> SRMQEKHMRIRVKLLDSTVELFDIEPKCDGQVLLTQVWKHLNLIECDYFGLEFKNVQSYWIWLEPMKPIIRQVRKPKNAVLRLAVKFFPPDPGQLQEEYTRYLFALQLKRDLLEERLTCTANTAALLISHLLQSEIGDYDETLDREHLKANEYLPNQEKSLEKILDFHQRHTGQTPAESDFQVLEIARKLEMYGIRFHMASDREGTKINLAVSHMGVLVFQGTTKINTFNWSKVRKLSFKRKRFLIKLHPEVHGPYQDTLEFLLGSRDECK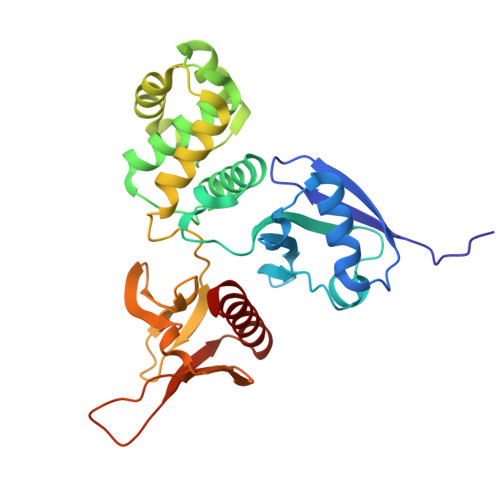NFWKICVEYHTFFRLSD> QYSPNTQQGRTSIVHLFEWRWVDIALECERYLAPKGFGGVQVSPPNENVAIYNPFRPWWERYQPVSYKLCTRSGNEDEFRNMVTRCNNVGVRIYVDAVINHMCGNAVSAGTSSTCGSYFNPGSRDFPAVPYSGWDFNDGKCKTGSGDIENYNDATQVRDCRLTGLLDLALEKDYVRSKIAEYMNHLIDIGVAGFQLDASKHMWPGDIKAILDKLHNLNSNWFPAGSKPFIYQEVIDLGGEPIKSSDYFGNGRVTEFKYGAKLGTVIRKWNGEKMSYLKNWGEGWGFVPSDRALVFVDNHDNQRGHGAGGASILTFWDARLYKMAVGFMLAHPYGFTRVM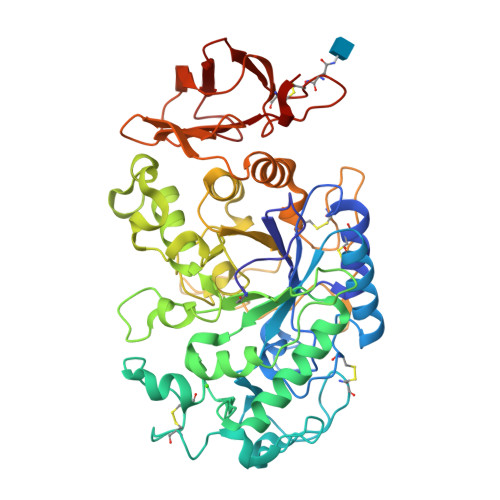SSYRWPRQFQNGNDVNDWVGPPNNNGVIKEVTINPDTTCGNDWVCEHRWRQIRNMVIFRNVVDGQPFTNWYDNGSNQVAFGRGNRGFIVFNNDDWSFSLTLQTGLPAGTYCDVISGDKINGNCTGIKIYVSDDGKAHFSISNSAEDPFIAIHAESKL>MEFIMKTRMFEEEGWIRKKCKVCGKPFWTLDPDRETCGDPPCDEYQFIGKPGIPRKYTLDEMREKFLRFFEKHEIYPHGRVKRYPVLPRWRDDVLLVGASIMDFQPWVISGEADPPANPLVISQPSIRFTDIDNVGITGRHFTIFEMMAHHAFNYPGKPIYWMDETVELAFEFFTKELKMKPEDITFKENPWAGGGNAGPAFEVLYRGLEVATLVFMQYKKAPENAPQDQVVVIKGEKYIPMETKVVDTGYGLERLVWMSQGTPTAYDAVLGYVVEPLKKMAGIEKIDEKILMENSRLAGMFDIEDLGDLRYLREQVAKRVGITVEELEKAIRPYELIYAIADHTKALTFMLADGVVPSNVKAGYLARLLIRKSIRHLRELGLEVPLSEIVALHIKELHKTFPEFKEMEDIILEMIELEEKKYAETLRRGSDLVRREIAKLKKKGIKEIPVEKLVTFYESHGLTPEIVKEIAEKEGVKVNIPDNFYSMVAKEAERTKEEKGEELVDFELLKDLPDTRRLYYEDPFMKEFDAKVLR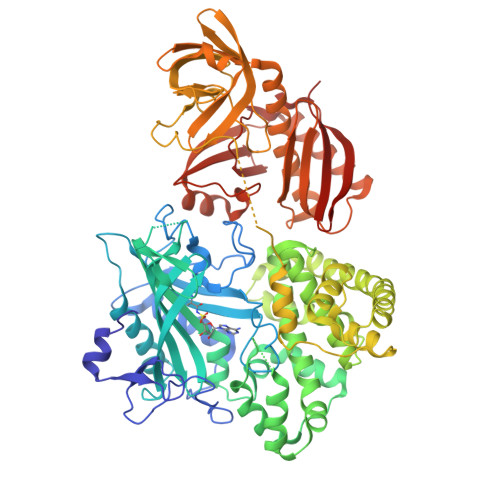VIKDWVILDATAFYPEGGGQPYDTGVLIVNGREVKVTNVQKVGKVIIHKVEDPGAFKEGMIVHGKIDWKRRIQHMRHHTGTHVLMGALVRVLGRHVWQAGSQLTTDWARLDISHYKRISEEELKEIEMLANRIVMEDRKVTWEWLPRTTAEQKYGFRLYQGGVVPGREIRVVKIEDWDVQACGGTHLPSTGLVGPIKILRTERIQDGVERIIFACGE[2x]>[8x]MENIMTLPKIKHVRAWFIGGATAEKGAGGGDYHDQGGNHWIDDHIATPMSKYRDYEQSRQSFGINVLGTLIVEV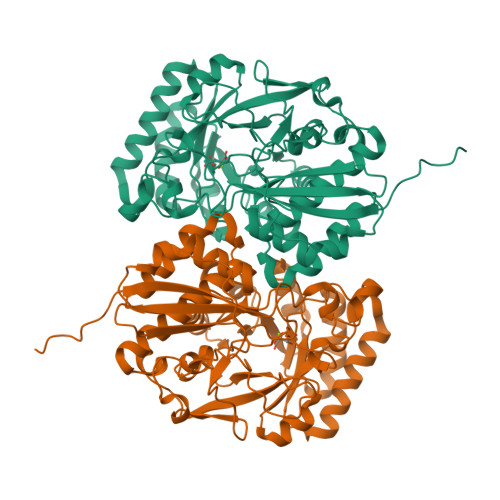EAENRQTGFAVSTAGEMGCFIVEKHLNRFIEGKCVSDIKLIHDQMLGATMYYSGSGGLVMNTISCVDLALWDLFGKVVGLPVYKLLGGAVRDEIQFYATGARPDLAKEMGFIGGKMPTHWGPHDGDAGIRKDAAMVADMREKCGPDFWLMLDCWMSQDVNYATKLAHACAPFNLKWIEECLPPQQYEGYRELKRNAPAGMMVTSGEHHGTLQSFRTLAETGIDIMQPDVGWCGGLTTLVEIAALAKSRGQLVVPHGSSVYSHHAVITFTNTPFSEFLMTSPDCSTLRPQFDPILLDEPVPVNGRIHKSVLDKPGFGVELNRDCHLKRPYSH(phenylmethyl) ~{N}-[(2~{S})-3-methyl-1-[[(2~{R})-1-[[(3~{R})-1-methylsulfanyl-4-oxidanylidene-pentan-3-yl]amino]-1-oxidanylidene-propan-2-yl]amino]-1-oxidanylidene-butan-2-yl]carbamate 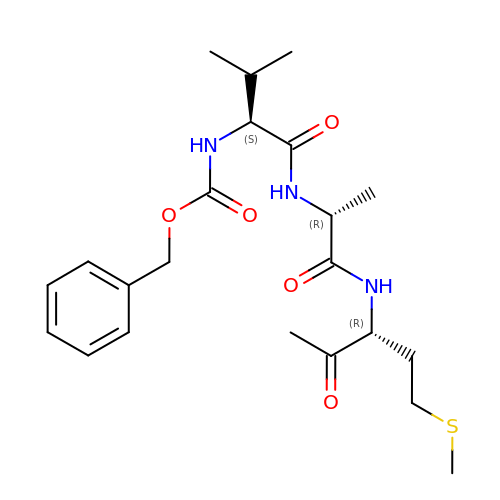| C22 H33 N3 O5 S | XQQSDBOJVLTWFC-LZQZEXGQSA-N> ART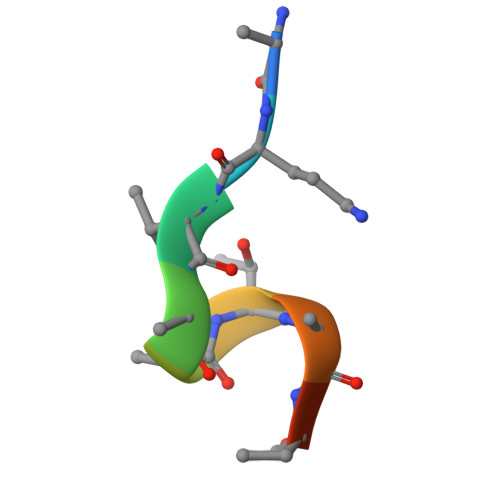AATARKS> EKKVGVIFGKFYPVHTGHINMIYEAFSKVDELHVIVCSDTVRDLKLFYDSKMKRMPTVQDRLRWMQQIFKYQKNQIFIHHLVEDGIPSYPNGWQSWSEAVKTLFHEKHFEPSIVFSSEPQDKAPYEKYLGLEVSLVDPDRTFFNVSATKIRTTPFQYWKFIPKEARPFFAKTVAILGGESSGKSVLVNKLAAVFNTTSAWEYGREFVFEKLGGDEQAMQYSDYPQMALGHQRYIDYAVRHSHKIAFIDTDFITTQAFCIQYEGKAHPFLDSMIKEYPFDVTILLKNNTEWVDDGLRSLGSQKQRQQFQQLLKK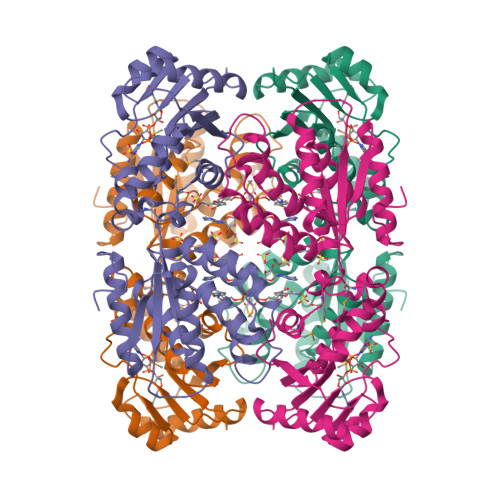LLDKYKVPYIEIESPSYLDRYNQVKAVIEKVLNEEEISELQNTTFPIKGTSQ>GQSTGQVTLGVLTDMSSVYADSAGKGSVAAVQLAIEDVGGKALGQPVKLVSADYQMKTDVALSIAREWFDRDGVDAIFDVVNSGTALAINNLVKDKKKLAFITAAAADQIGGTECNGYGIGFLYNFTSIVKTVVQAQLAKGYKTWFLMLPDAAYGDLMNAAIRRELTAGGGQIVGSVRFP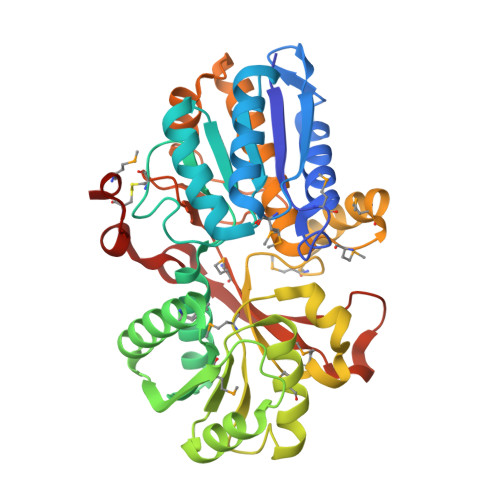FETQDFSSYLLQAKASGAQLIVSTSGGAANINIMKQAREFGLPSKTQKVGGMIDILTDVKSAGLRVMQGQEYATSFYWNMDDRTRAFAKRFYAKMGKMPTNNQAGGYSAALQYLKAVNAIGSKDPQKVFAYLKTIKFDDAVTRHGTLRPGGRLVRDMYLVRAKKPEDQKGDWDYYDVVATIGPEQAFGPLSESRCAMDK[2x]>[2x]NYLDLFSHKNMKL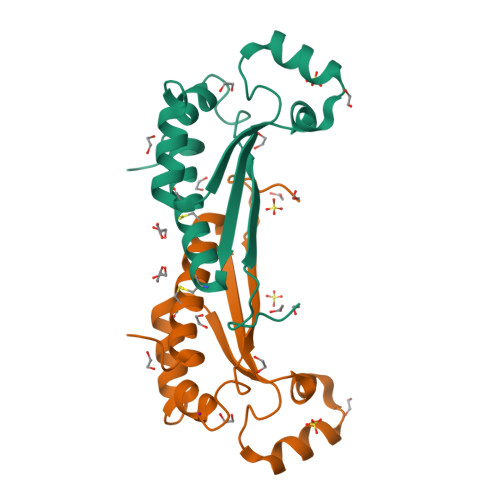KERVLIPVKQYPKFNFVGKILGPQGNTIKRLQEETGAKISVLGKGSMRDKAKEEELRKGGDPKYAHLNMDLHVFIEVFGPPCEAYALMAHAMCEVKKFLVPDMMD> HQDKVPCKMVDKKVSCQVLGLLQVPSVLPPDTETLDLSGNQLRSILASPLGFYTALRHLDLSTNEISFLQPGAFQALTHLEHLSLAHNRLAMATALSAGGLGPLPRVTSLDLSGNSLYSGLLERLLGEAPSLHTLSLAENSLTRLTRHTFRDMPALEQLDLHSNVLMDIEDGAFEGLPRLTHLNLSRNSLTCISDFSLQQLRVLDLSCNSIEAFQTASQPQAEFQLTWLDLRENKLLHFPDLAALPRLIYLNLSNNLIRLPTGPPQDSKGIHAPSEGWSALPLSAPSGNASGRPLSQLLNLDLSYNEIELIPDSFLEHLTSLCFLNLSRNCLRTFEARRLGSLPCLMLLDLSHNALETLELGARALGSLRTLLLQGNALRDLPPYTFANLASLQRLNLQGNRVSPC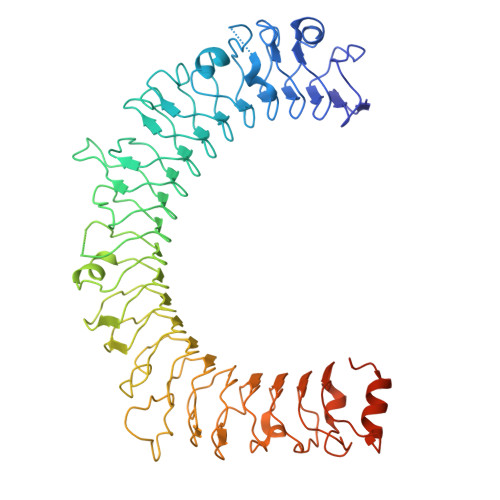GGPDEPGPSGCVAFSGITSLRSLSLVDNEIELLRAGAFLHTPLTELDLSSNPGLEVATGALGGLEASLEVLALQGNGLMVLQVDLPCFICLKRLNLAENRLSHLPAWTQAVSLEVLDLRNNSFSLLPGSAMGGLETSLRRLYLQGNPLSCCGNGWLAAQLHQGRVDVDATQDLICRFSSQEEVSLSHVRPEDCEKGGLKNIN> MAHHHHHHMPTQAVDDLIHILLVEDSPTDVMITREAFDYYKLLNPLHVAGDGVAAMEFLRREGQHSDAPRPGLIILDLNLPKKSGREVLQELKADPDLMKIPVVVLTTSKSEEDVA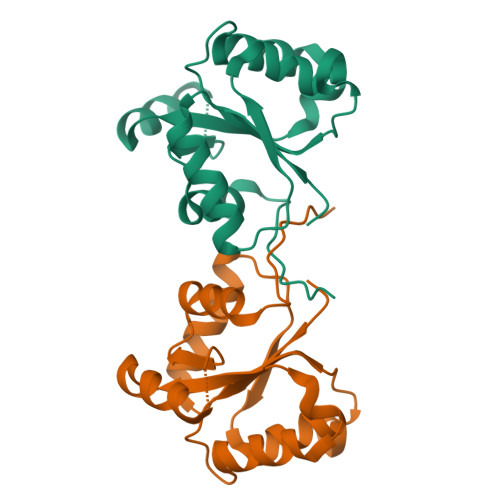RTYGLHANCYITKPVDFTRFVEVVRRISDFWFGVVTLPPARS>MSQVDINPARALVYQLLSSLFAREVDEQRLKELTSEAAQQFWEQLSLEANFTQSVDKIRSTLNGIKDDEALLELAADYCGLFLVGTKHSASPYASLYLSGEDEPLLFGEQHQQMSEFLHQSKLQVQSHFPE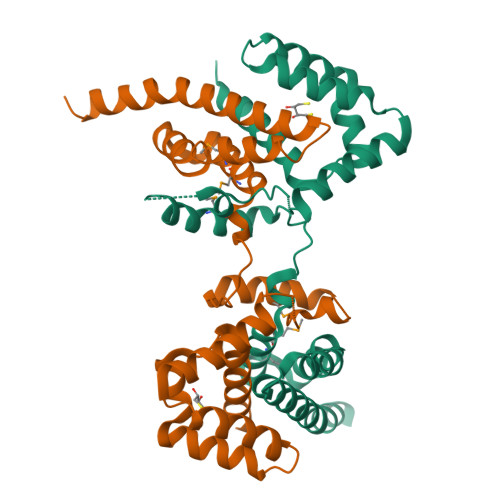PADHLAVMLAYMAHLCCHSENSVQLSFLQTCVNSWLAKFINHLTQCNKNGFYSAVATLTLAWVKQDIAQLEPAVAIISLEHHHHHH[2x]> LYKKAGFMKGIYSA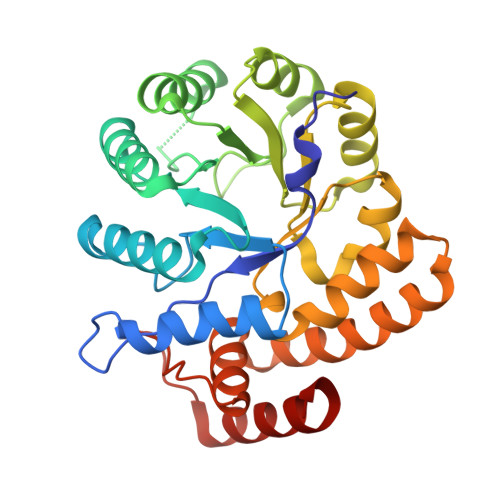LMVPYNEDGSINEKGLREIIRYNIDKMKVDGLYVGGSTGENFMISTEEKKRVFEIAIDEAKDSVNLIAQVGSINLNEAVELGKYVTKLGYKCLSAVTPFYYKFDFSEIKDYYETIVRETGNYMIIYSIPFLTGVNMSLSQFGELFENEKIIGVKFTAGDFYLLERVRKAFPDKLIFAGFDEMLLPATVLGVDGAIGSTYNINGIRAKQIFELAKNSKIDEALKIQHTTNDLIEGILSNGLYQTIKEILKLEGVDAGYCRKPMKKISQKQIEFAKELHKKFLK>MSGDN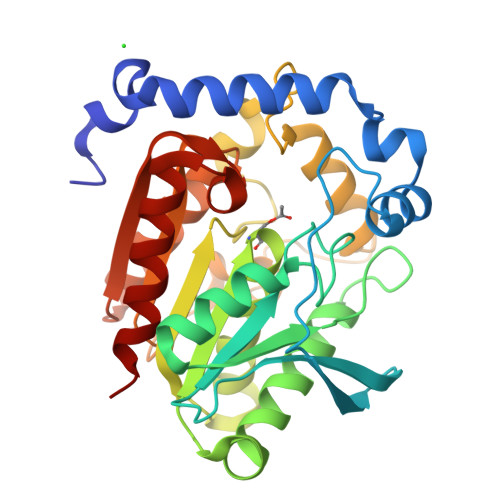PFDPELYKDAAVSAETRALNTALIDLLETSDDNWDIGVEEARARRDRGEGPFPAVPKSPRARTIQIPGKGGDIALRIIAPETPKGVYLHFHGGGWVFGSADGQDPMLERISDTTGLVCVSVEYRLAPEHPYPAGPDDCESAALWLVENAKREFGTDLLTIGGESAGGHLAAVTLLRMRDRHGFTGFAGANLVFGAFDLRWTPSARSYGNDRYLILRTLDLEKFDACFLPENVDRADPDISPLMANLHDMPPALFTVGTDDALLDDSLFMHARWAAAGNEAELAVYPGGAHGFVAFPGALAASAVQRMDAFLKRFTD[4x]3-(2-imidazo[1,2-b]pyridazin-3-ylethynyl)-4-methyl-~{N}-[4-(propanoylamino)-3-(trifluoromethyl)phenyl]benzamide | C26 H20 F3 N5 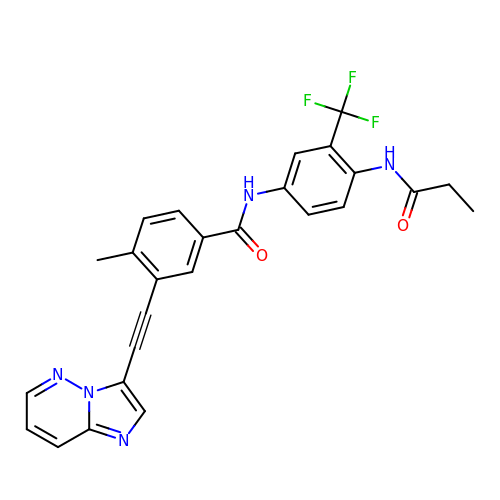O2 | FTNOFDRVSQZWOA-UHFFFAOYSA-N4-[3-azanyl-6-[1-methyl-5-(1-phenylcyclopropyl)-1,2,4-triazol-3-yl]pyrazin-2-yl]pyrazole-1-carboxamide | C20 H19 N9 O | 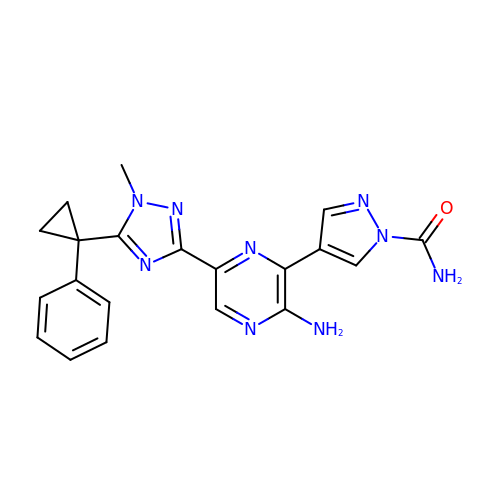FIICMSQLNYXQBM-UHFFFAOYSA-N>[7x]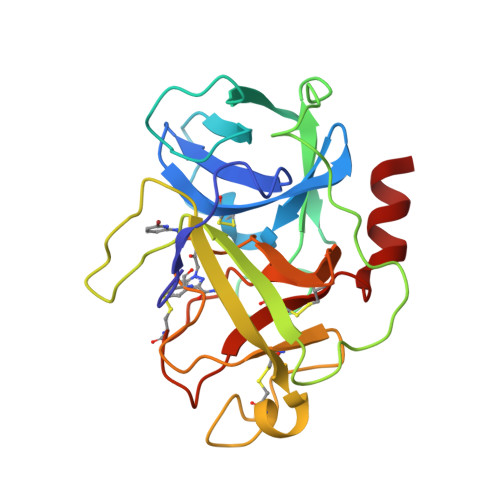ILGGREAEAHARPYMASVQLNGAHLCGGVLVAEQWVLSAAHCLEDAADGKVQVLLGAHSLSQPEPSKRLYDVLRAVPHPDSQPDTIDHDLLLLQLSEKATLGPAVRPLPWQRVDRDVAPGTLCDVAGWGIVNHAGRRPDSLQHVLLPVLDRATCNRRTHHDGAITERLMCAESNRRDSCKGDSGGPLVCGGVLEGVVTSGSRVCGNRKKPGIYTRVASYAAWIDSVLA> 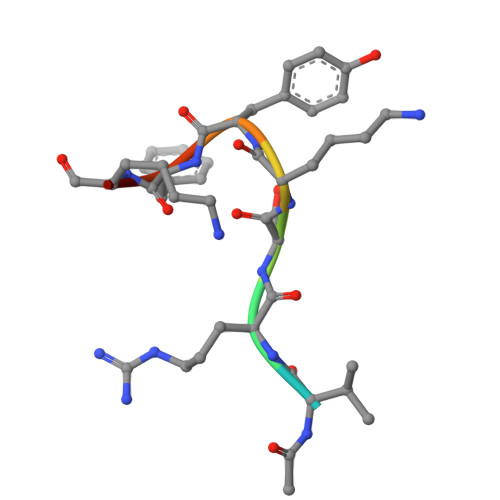XVRSKYFKK>MILNNQEWLLAIFKKKGLTPTGKLEFATIDGIDSALAQALNEAFDSQVVSFNDRINQSFREFLKRTPRDRITLGTFSDVKEWLSSFEADRAGRKDTASAGPVNKLAMPLVNLSRSPAFSIYEGELCRDNYDEGHVTNENDEIEALVSTIPFSLEYSLWIASDEKESLGMVTTALAFWLRMYASLGQASFTHIANVGGYEIPVTCYIEGQKSIAFQDLTTGTADNRLFAVGLNLTVVAELPILAYMQQTTGTITVKAKILEE[6x];>MGHNNTKGNRKFIKGRYTANAAKGERLVSSEFLLTFAGHEDISVLVRTSQIPEMTREDVEDYGPNGVKFNQHGPIRNSGEIQVQCVETIEGDILQFIKDRIAAKDYVDITMAATPESKSSGVNAVTKAATTIEMLDCKIYSDAIDFSTEDVTAAVRPSLRIVYNWIEWD[12x];>[12x]MSQYSIQQSLGNASGVAVSPINADATLSTGVALNSSLWAGIGVFARGKPFTVLAVTESNYEDVLGEPLKPSSGSQFEPIRHVYEAIQQTSGYVVRAVPDDAKFPIIMFDESGEPAYSALPYGSEIELDSGEAFAIYVDDGDPCISPTRELTIETATADSAGNERFLLKLTQTTSLGVVTTLETHTVSLAEEAKDDMGRLCYLPTALEARSKYLRAVVNEELISTAKVTNKKSLAFTGGTNGDQSKISTAAYLRAVKVLNNAPYMYTAVLGLGCYDNAAITALGKICADRLIDGFFDVKPTLTYAEALPAVEDTGLLGTDYVSCSVYHYPFSCKDKWTQSRVVFGLSGVAYAAKARGVKKNSDVGGWHYSPAGEERAVIARASIQPLYPEDTPDEEAMVKGRLNKVSVGTSGQMIIDDALTCCTQDNYLHFQHVPSLMNAISRFFVQLARQMKHSPDGITAAGLTKGMTKLLDRFVASGALVAPRDPDADGTEPYVLKVTQAEFDKWEVVWACCPTGVARRIQGVPLLIK

The phage tail is a macromolecular machine responsible for specifically recognizing host bacteria, penetrating the cell membrane, and forming a channel for genome delivery. The conserved structural components include three main parts: a baseplate, a long inner tail tube, and a tail sheath that wraps around the tube. Phage P1, a temperate phage first discovered in 1951, transfers DNA into a wide range of gram-negative bacterial species by universal transduction and has been used to construct a fine structural genetic map of E. coli. During the tail-contraction, the tail sheath undergoes a massive conformational change and contracts to half and more of its original length, exposing the inner tail tube and providing the energy to drive the tail tube to eventually penetrate the target cell membrane.

To improve the reconstruction resolution, we then re-boxed sub-particles and resolved the partial structure of the P1 extended tail, including a tail terminator ring, eight sixfold sheath rings, and eight sixfold tube rings at 3.3 Å resolution, which allowed us to build the atomic models for the tail terminator protein gp24, the tail tube protein BplB, and the tail sheath protein gp22. The 53-layer tail sheath and tube of phage P1 are terminated by a hexameric terminator that covers the distal inner tail tube and embraces the top ring of the sheath. The terminator consists of six copies of protein gp24, and each gp24 consists of four domains: a central core domain (residues 23–127, 151–244), a β-hairpin domain (residues 128–150), an N-terminal domain (residues 2–22), and a C-terminal domain (residues 245–260). The inserted β-hairpin domain extends into the distal ring of the tail tube and lies in a groove formed by two adjacent tail tube subunits, and these interactions result in the tail tube protein in the top layer having a different conformation than that in the other layers. The N-terminal and C-terminal domains of each gp24 together form a two-antiparallel-stranded β-sheet that is inserted into the top ring of the sheath to form an augmenting β-sheet. The 169-residue tail tube protein BplB consists of a β-sandwich domain flanked by an α-helix and an extended N-terminal domain (residues 1–31) arranged in an α-helix and two loops. The β-hairpin plug of one ring is precisely inserted into the N-terminal outer rim of the adjacent ring exactly, and relies on the electrostatic interactions between the plug and rim to form a stable 53-ring tail tube. First, the N-terminal α-helix transforms into a β-strand that interacts with the β-hairpin domain of the terminator protein gp24 by β-sheet augmentation.> MGEETI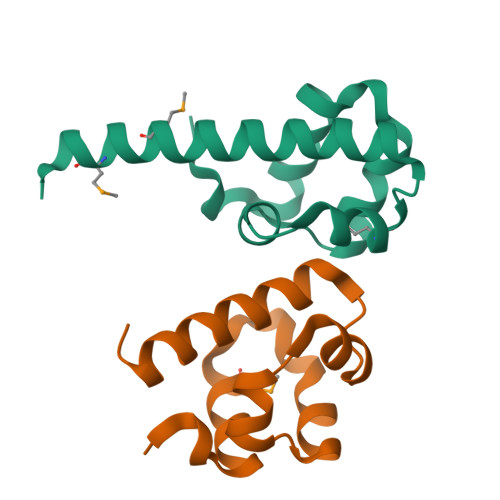NSTQNKTRTKTTRPKAVYLWTVSDVLKWYRRHCGEYTQYEQLFAQHDITGRALLRITDSSLQRMGVTDNRDREAIWREIVKQRLKTDIMEIRDMERLNIY;> MEPVSKWSPSQVVDWMKGLDDCLQQYIKNFEREKISGDQLLRITHQELEDLGVSRIGHQELILEAVDLLCALNYGLETEN>[5x]MSEWSRIAVEFGEQQLNLTELEDFARELAYEGLDPALIIKKLKETGG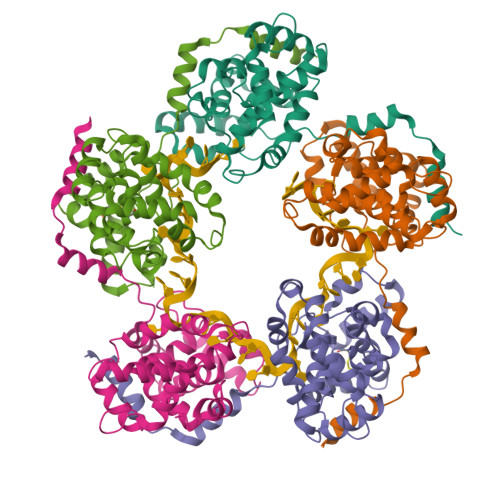DDWVKDTKFIIVFALTRGNKIVKASGKMSNSGSKRLMALQEKYGLVERAETRLSITPVRVAQSLPTWTCAAAAALKEYLPVGPAVMNLKVENYPPEMMCMAFGSLIPTAGVSEATTKTLMEAYSLWQDAFTKTINVKMRGASKTEVYNSFRDPLHAAVNSVFFPNDVRVKWLKAKGILGPDGVPSRAAEVAAAAYRNL> MEDPVTGPEEVSGQEQGSLTVQCRYTSGWKDYKKYWCQGVPQRSCKTLVETDASEQLVKKNRVSIRDNQRDFIFTVTMEDLRMSDAGIYWCGITK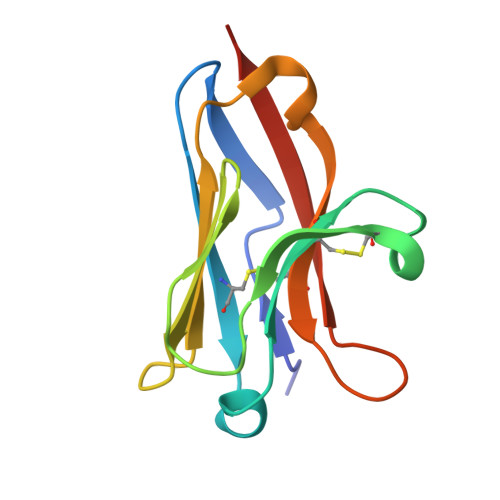GGLDPMFKVTVNIGPVPT>EEAELAYLLGELAYKLGEYRIAIRAYRIALKRDPNNAEAWYNLGNAYYKQGDYDEAIEYYQKALELDPNNAEAWYNLGNAYYKQGDYDE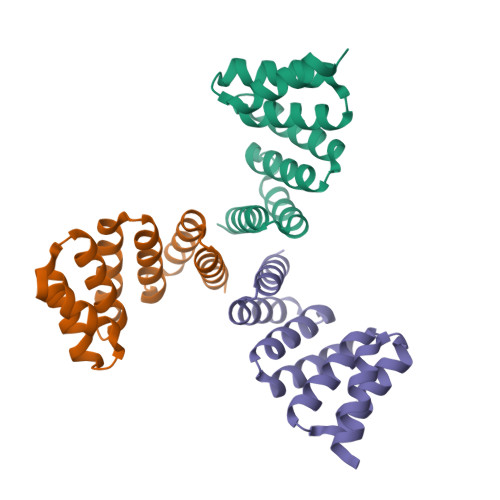AIEYYQKALELDPNNAEAKQNLGNAKQKQG[6x]5-hydroxy-N-(4-oxo-3H-quinazolin-6-yl)-1-[3-[(phenylcarbamoylamino)methyl]phenyl]pyrazole-4-carboxamide | C26 H21 N7 O4 | 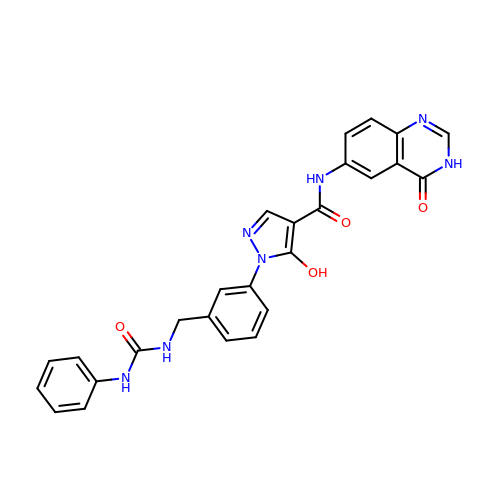TVWGVVMNUMHISA-UHFFFAOYSA-N6-methoxy-2-(1H-pyrazol-5-yl)-1H-benzimidazole | C11 H10 N4 O | 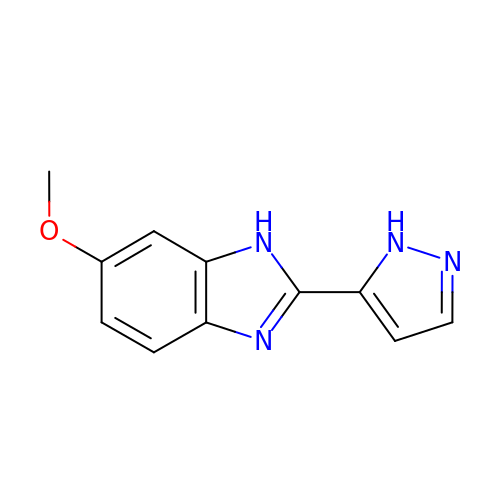KSQSJEOPBMYGOB-UHFFFAOYSA-N>GLVPRGSHMKKLLVANRGEIAVRVFRACNELGLSTVAVYAREDEYSVHRFKADESYLIGQGKKPIDAYLDIDDIIRVALESGADAIHPGYGLLSENLEFATKVRAAGLVFVGPELHHLDIFGDKIKAKAAADEAKVPGIPGTNGAVDIDGALEFAKTYGYPVMIKAALGGGGRGMRVARNDAEMHDGYARAKSEAIGAFGSGEIYVEKYIENPKHIEVQILGDRHGNIIHLHERDCSVQRRNQKVIEIAPAVGLSPDFRNEICEAAVKLCKNVGYVNAGTVEFLVKDDKFYFIEVNPRVQVEHTITELITGVDIVQAQILIAQGKDLHREIGLPAQSEIPLLGSAIQCRITTEDPQNGFLPDTGKIDTYRSPGGFGIRLDVGNAYAGYEVTPYFDSLLVKVCTFANEFSDSVRKMDRVLHEFRIRGVKTNIPFLINVIANENFTSGQATTTFIDNTPSLFNFPRLRDRGTKTLHYLSMITVNGFPGIENTEKRHFEEPRQPLLNLEKKKTAKNILDEQGADAVVDYVKNTKEVLLTDTTLRDAHQSLLATRLRLQDMKGIAQAIDQGLPELFSAEMWGGATFDVAYRFLNESPWYRLRKLRKLMPNTMFQMLFRGSNAVGYQNYPDNVIEEFIRVAAHEGIDVFRIFDSLNWLPQMEKSIQAVRDNGKIAEATICYTGDILDPSRPKYNIQYYKDLAKELEATGAHILAVKDMAGLLKPQAAYRLISELKDTVDLPIHLHTHDTSGNGIITYSGATQAGVDIIDVATASLAGGTSQPSMQSIYYALEHGPRHASINVKNAEQIDHYWEDVRKYYAPFEAGITSP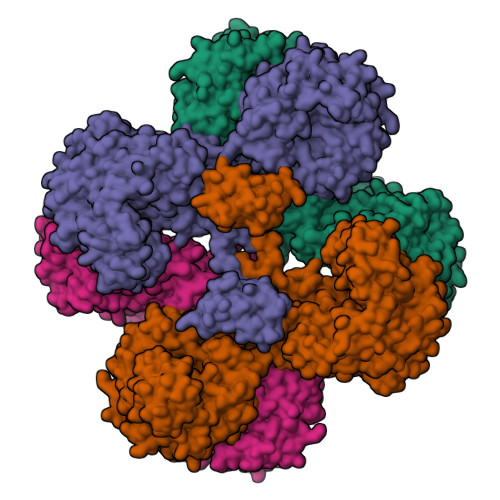QTEVYMHEMPGGQYTNLKSQAAAVGLGHRFDEIKQMYRKVNMMFGDIIKVTPSSKVVGDMALFMIQNDLTEEDVYARGNELNFPESVVSFFRGDLGQPVGGFPEKLQKIIVKDKAVITDRPGLHAEKVDFETVKADLEQKIGYEPGDHEVISYIMYPQVFLDYQKMQREFGAVTLLDTPTFLHGMRLNEKIEVQIEKGKTLSIRLDEIGEPDLAGNRVLFFNLNGQRREVVINDQSVQAQVVAKRKAETGNPNQIGATMPGSVLEILVKAGDKVQKGQALMVTEAMKMETTIEAPFDGEIVDLHVVKGEAIQTQDLLIEIN[4x]>AKKIILDCDPGLDDAVAILLAHGNPEIELLAITTVVGNQTLAKVTRNAQLVADIAGITGVPI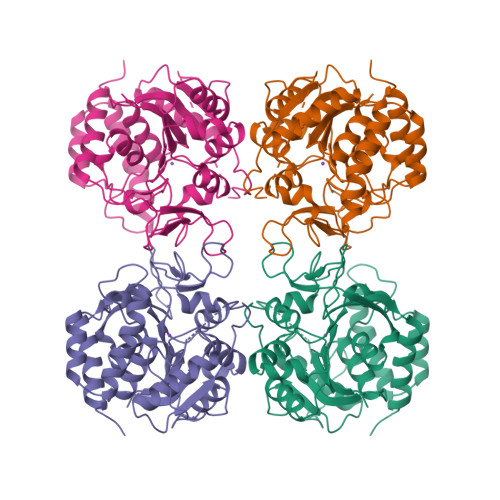AAGCDKPLVRKIMTAGHIHGESGMGTVAYPAEFKNKVDERHAVNLIIDLVMSHEPKTITLVPTGGLTNIAMAARLEPRIVDRVKEVVLMGGGYHEGNATSVAEFNIIIDPEAAHIVFNESWQVTMVGLDLTHQALATPPILQRVKEVDTNPARFMLEIMDYYTKIYQSNRYMAAAAVHDPCAVAYVIDPSVMTTERVPVDIELTGKLTLGMTVADFRNPRPEHCHTQVAVKLDFEKFWGLVLDALERIGDPQ[2x]> EERKKELAKEVIETAK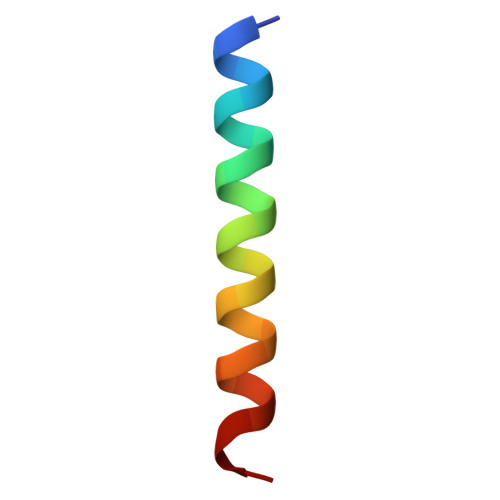KLIEKLAKEE Carbohydrate-binding modules (CBMs) are non-catalytic proteins found appended to carbohydrate-active enzymes. Soil and marine bacteria secrete such enzymes to scavenge nutrition, and they often use CBMs to improve reaction rates and retention of released sugars. Here we present a structural and functional analysis of the recently established CBM family 92. All proteins analysed bind preferentially to β−1,6-glucans.

Soaking experiments of the CpCBM92B protein crystals with glucose, gentiobiose (G2: Glc-β-1,6-Glc), and sophorose (S2: Glc-β−1,2-Glc) revealed a binding cleft within each subdomain comprising a Trp-Glu binding motif, again implying three polysaccharide binding sites per protein. In each ligand complex, the glucosyl unit stacks with the conserved Trp with the O3 and O4 of the sugar positioned by hydrogen bonding with the Oε1 and Oε2 of the conserved Glu. In the binding site of CpCBM92B subdomain β, the protein is observed to further interact with the glucosyl unit through the guanidine group of Arg955 with the O2 of the sugar, and through the carbonyl of a succinimide formed in place of Asp959 with the sugar O6. Indeed, only 45 protein entries containing this chemical group are currently reported in the PDB45. In our investigation it was found only in the β-subdomain of CpCBM92B and it may be an artefact of protein production or crystallisation. Collectively, the binding modes observed with the ligand complexes reveal the possibility for extensions from both the O1 and O6, presumably enabling binding along a β−1,6-glucan chain such as in pustulan, and additionally binding to β-1,6-linked glucosyl substitutions in, for example, scleroglucan or laminarin. The crystal structures with glucose-based ligands provide evidence for chain-end binding to the non-reducing end of a ligand, with space for potential extension at O2 and O6, which would additionally permit mid-chain binding to glycans with those linkages. According to the crystal structures, mid-chain binding to e.g. β−1,3-glucan or β-1,4-glucan would not be possible.

>[2x]MASMTGGQQMGRGSKTIWLQGFNSKYVNSRNGQGAMWCDSDTPQAWELFTVIDAGNGKIALRGNNGLYVSSENGEQAMTCNRPAINGWEVFDWISNSDGSVSLRGSNGMYVSSENGEQAITCNRPAIDGWERFNWAAATLEHHHHHH> GHMLGSGFKAERLRVNLRLVINRLKLLEKKKTELAQKARKEIADYLAAGKDERARIRVEHIIREDYLVEAMEILELYCDLLLARFGLIQSMKELDSGLAESVSTLIWAAPRLQSEVAEL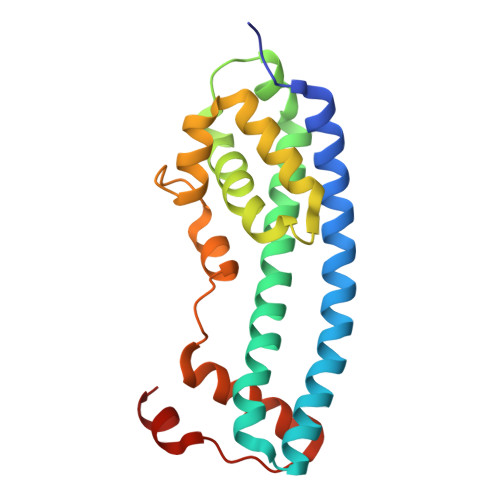KIVADQLCAKYSKEYGKLCRTNQIGTVNDRLMHKLSVEAPPKILVERYLIEIAKNYNVPYEPDSVVMAEAPP> MDYQEALLELIERLLRKLNVDPRDIKRIEQQLRDLDIYQIALLLLI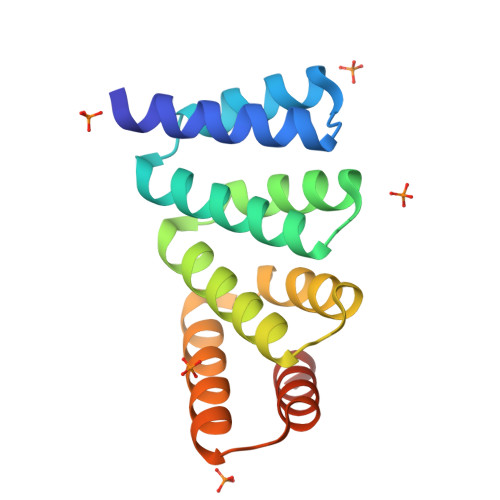ILLLRKLNVDPRDIKRILQQLIDLDIYQIALLLLIILLLHKLNVDPRDIKRILQQLIDLDIEQIAELLLRILELRKRNEDPRDIKRELQQLIDDDGSWLE> GPTAAALEPHPEEKKKKRSGFRDRKVMEYENRIRAYSTPDKIFRYFATLKVISEPGEAEVFMTPEDFVRSITPNEKQPEHLGLDQYIIKRFDGKKISQEREKFADEGSIFYTLGECGLISFSDYIFLTTVLSTPQRNFEIAFKMFDLNGDGEVDMEEFEQVQSIIRSQTSMGMRHRDRPTTGNTLKSGLCSALTTYFFGADLKGKLTIKNFLEFQRKLQHDVL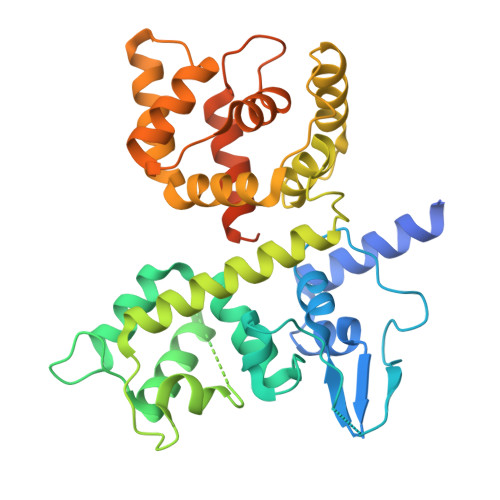KLEFERHDPVDGRITERQFGGMLLAYSGVQSKKLTAMQRQLKKHFKEGKGLTFQEVENFFTFLKNINDVDTALSFYHMAGASLDKVTMQQVARTVAKVELSDHVCDVVFALFDCDGNGELSNKEFVSIMKQRLMRGLEKPKDMGFTRLMQAMWKCAQETAWDFALPKQSNW> SQCKAMTVKFTVELDIERLTGQTYTDFIKNLRRSLATWYLHGVPVLPLYNQEADPRGFDLKLTFRGQVTTVRIHRDDLVLRGYQMQGAGKWLELERPSTQTGHLIEGSELLEFGPSYEELAAAAQQDILDISYNKNALQDAVSKLAVSTNTRDRARSLIVVSQMFCEATRFVDIANHFAFNLESSEPVKLPQWMQNDLEKNWVRFSFMILKSNADPCYKFEPQTIY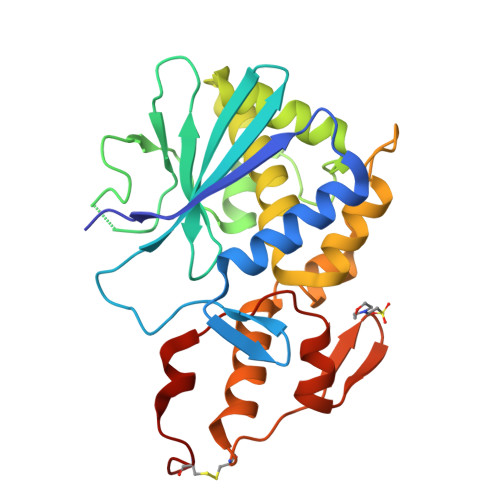GKIIKTADELLNFLGIVEQHPDTRSPPCAAG>[26x]MAYAQWVIIIIHNVGSQDVKIKNLKASWGKLHADGDKDAEVSASNYEGKIVKPDEKLQINASGRSDAAEGTTGTFDLVDPADGDKQVRHFYWDSPWG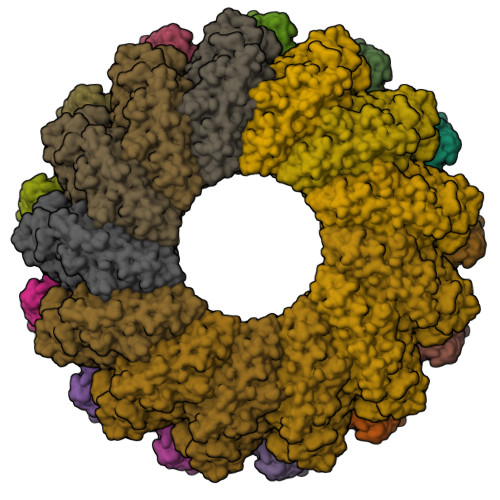SKTNTWTVSGSNTKWMIEYSGQNLDSGALGTITVDTLKKGENLYFQ;>[13x]HHHHHHHHSQAGDTLNDVIQDPTRRNKLINDNNLLKGIIMGRDGPVPSSRELIVRPDTLRAIINNRATIETTTMEAEFTETLMESNYNSASVKVSAPFITANSEYSESSSFKNTETEKSMYTSSRYLFPQGRIDFTTPDSGFDDVIKLSPQFTSGVQAALAKATGTEKREALQNLFQEYGHVFRTKVHIGGVLSAHTMETFSRSENETEVKQDVKAGLEGAVKGWGGGATAGHGNTQGTITTSQNRKLNVKYIVNVVDYTKIQNTEEWVASTNQSEHWRVIEVTEVTAVADLLPQPIRGQVKDLLKPLLGKWVDVEKVPGLESLPVSVYRPKGAIPAGWFWLGDTADASKALLVKPTLPARSGRNPALTSLHQGSGMTEQPFVDLPQYQYLSTYFGSFAHDTPPGSTLRGLRPDHVLPGRYEMHGDTISTAVYVTRPVDVPFPEDECFDLKSLVRVKLPGSGNPPKPRSALKKSMVLFDSGEK>SAIAGMSSEYVPPKVWKWDKANGGAFASVNRPVAGPTSERELPVGKHPFQVYSLGTPNGQKATIMLEELLQLGFSEAEYDAWLIKIFEGDQFTSGFVDINPNSKIPAMVDRSGPEPFRVFESGAILMHLAEKFGVFLPTSGPARAECLSWLFWQVGSAPFIGGGFGHFYNYAPIKIEYAIDRYAMETKRLFDVANRRLAESRYLAGDEYTIADLATYTWFGNIYRGEAYGEAATFLSMHEYEHVGRWVGEIDARPGVLRGRLVNSSKG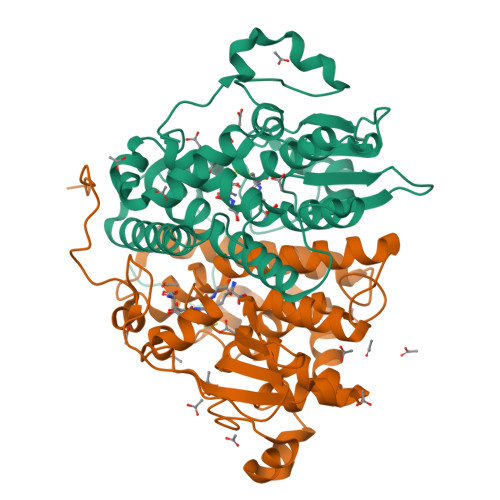LAERHDASDFDALPPESLQAIVKGF[2x]> GAMGENEKLINKIGPNIEMFAQTINTDIQKIEPNDQFGINKTLFTEKKDNNIDFMLKDNRLRRLFYSSLNYDENKIKKLATILAQTSSSNDYHYTLIGLIFWTGFKIQEAFESAVNILTKDE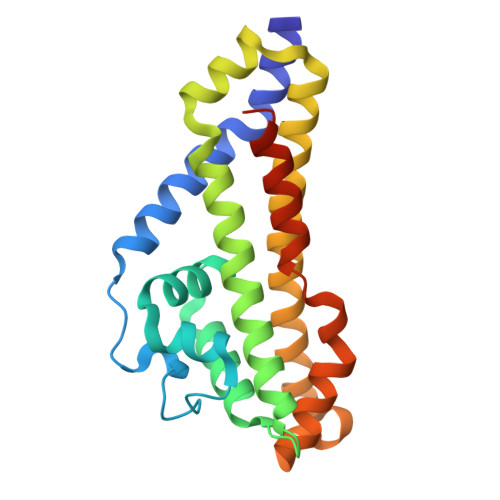QKRLIFNFRTKTVKEIQENFEKLMQERNSWIKIVDNIIGEYDKNTGGCKADGKILGEVIRVGYEHELDSNKSMQILNNIETPLKTCCDHIHY>GSHMASMTGGQQMGRGSMSKIVKIIGREIIDSRGNPTVEAEVHLEGGFVGMAAAPSGASTGSREALELRDGDKSRFLGKGVTKAVAAVNGPIAQALIGKDAKDQAGIDKIMIDLDGTENKSKFGANAILAVSLANAKAAAAAKGMPLYEHIAELNGTPGKYSMPVPMMNIINGGEHADNNVDIQEFMIQPVGAKTVKEAIRMGSEVFHHLAKVLKAKGMNTAVGDEGGYAPNLGSNAEALAVIAEAVKAAGYELGKDITLAMDCAASEFYKDGKYVLAGEGNKAFTSEEFTHFLEELTKQYPIVSIEDGLDESDWDGFAYQTKVLGDKIQLVGDDLFVTNTKILKEGIEKGIANSILIKFNQ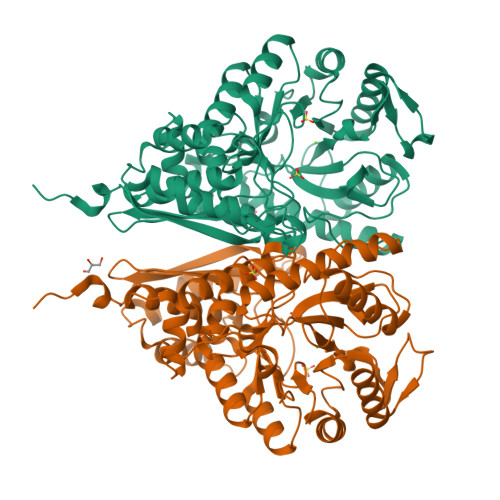IGSLTETLAAIKMAKDAGYTAVISHRSGETEDATIADLAVGTAAGQIKTGSMSRSDRVAKYNQLIRIEEALGEKAPYNGRKEIKGQA[6x]>SRKTYTLTDYLKNTYRLKLYSLRWISDHEYLYKQENNILVFNAEY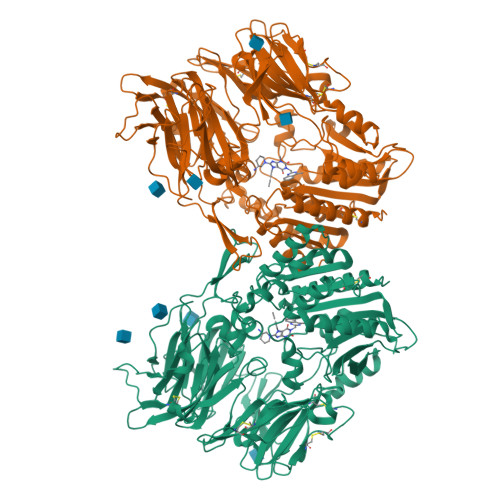GNSSVFLENSTFDEFGHSINDYSISPDGQFILLEYNYVKQWRHSYTASYDIYDLNKRQLITEERIPNNTQWVTWSPVGHKLAYVWNNDIYVKIEPNLPSYRITWTGKEDIIYNGITDWVYEEEVFSAYSALWWSPNGTFLAYAQFNDTEVPLIEYSFYSDESLQYPKTVRVPYPKAGAVNPTVKFFVVNTDSLSSVTNATSIQITAPASMLIGDHYLCDVTWATQERISLQWLRRIQNYSVMDICDYDESSGRWNCLVARQHIEMSTTGWVGRFRPSEPHFTLDGNSFYKIISNEEGYRHICYFQIDKKDCTFITKGTWEVIGIEALTSDYLYYISNEYKGMPGGRNLYKIQLSDYTKVTCLSCELNPERCQYYSVSFSKEAKYYQLRCSGPGLPLYTLHSSVNDKGLRVLEDNSALDKMLQNVQMPSKKLDFIILNETKFWYQMILPPHFDKSKKYPLLLDVYAGPCSQKADTVFRLNWATYLASTENIIVASFDGRGSGYQGDKIMHAINRRLGTFEVEDQIEAARQFSKMGFVDNKRIAIWGWSYGGYVTSMVLGSGSGVFKCGIAVAPVSRWEYYDSVYTERYMGLPTPEDNLDHYRNSTVMSRAENFKQVEYLLIHGTADDNVHFQQSAQISKALVDVGVDFQAMWYTDEDHGIASSTAHQHIYTHMSHFIKQCFSLPHHHHHH[2x]> QI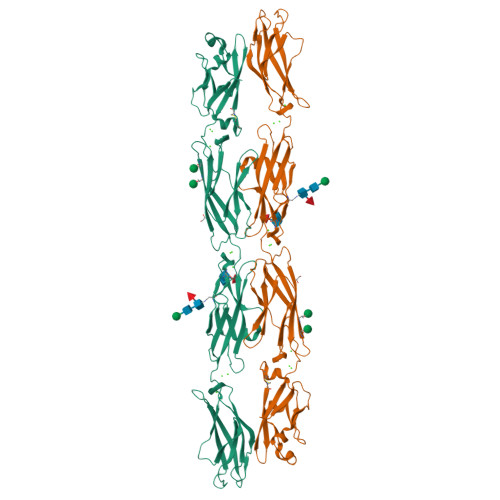RYPVPEESQEGTFVGNVAQDFLLDTESLSARRLQVAGEVNQRHFRVDLDSGALLIKNPIDREALCGLSASCIVPLEFVTEGPLEMYRAEVEIVDVNDHAPRFPRQQLDLEIGEAAPPGQRFPLEKAQDADVGSNSISSYRLSSNEHFALDVKKRSDGSLVPELLLEKPLDREKQSDYRLVLTAVDGGNPPRSGTAELRVSVLDVNDNAPAFQQSSYRISVLESAPAGMVLIQLNASDPDLGPSGNVTFSFSGHTPDRVRNLFSLHPTTGKLTLQGPLDFESENYYEFDVRARDGGSPAMEQHCSLRVDLLDVNDNAPHITVTSELGTLPESAEPGTVVALISVQDPDSGSNGDVSLRIPDHLPFALKSAFRNQFSLVTAGPLDREARSSYDIMVTASDAGNPPLSTHRTIFLNISDVNDHHHHHHHH>[4x]MSEKNVSIVVAASVLSSGIGINGQLPWSISEDLKFFSKITNNKCDSNKKNALIMGRKTWDSIGRRPLKNRIIVVISSSLPQDEADPNVVVFRNLEDSIENLMNDDSIENIFVCGGESIYRDALKDNFVDRIYLTRVALEDIEFDTYFPEIPETFLPVYMSQTFCTKNISYDFMIFEKQEKKTLQNCDPARGQLKSIDDTVDLLGEIAGIRKMGNRHKFPKEEIYNTPSIRFGREHYEFQYLDLLSRVLENGAYRENRTGISTYSIFGQMMRFDMRESFPLLTTKKVAIRSIFEELIWFIKGDTNGNHLIEKKVYIWSGNGSKEYLERIGLGHREENDLGPIYGFQWRHYNGEYKTMHDDYTGVGVDQLAKLIETLKNNPKDRRHILTAWNPSALSQMALPPCHVLSQYYVTNDNCLSCNLYQRSCDLGLGSPFNIASYAILTMMLAQVCGYEPGELAIFIGDAHIYENHLTQLKEQLSRTPRPFPQLKFK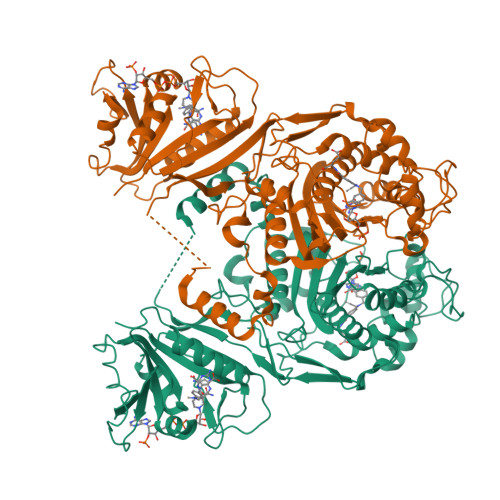RKVENIEDFKWEDIELIGYYPYPTIKMDMAV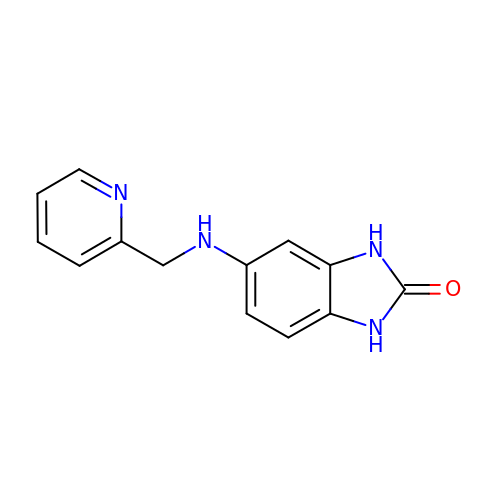5-[(pyridin-2-ylmethyl)amino]-1,3-dihydro-2H-benzimidazol-2-one | C13 H12 N4 O | MRKXGDLFRQWMOW-UHFFFAOYSA-N>MGSSHHHHHHSSGENLYFQGHMMDLTVEPNLHSLITSTTHKWIFVGGKGGVGKTTSSCSIAIQMALSQPNKQFLLISTNPAHNLSDAFGEKFGKDARKVTGMNNLSCMEIDPSAALKDMNDMAVSRANNNGSDGQGDDLGSLLQGGALADLTGSIPGIDEALSFMEVMKHIKRQEQGEGETFDTVIFDTAPTGHTLRFLQLPNTLSKLLEKFGEITNKLGPMLNSFMGAGNVDISGKLNELKANVETIRQQFTDPDLTTFVCVCISEFLSLYETERLIQELISYDMDVNSIIVNQLLFAENDQEHNCKRCQARWKMQKKYLDQIDELYEDFHVVKMPLCAGEIRGLNNLTKFSQFLNKEYNPITDGKVIYELEDKE[2x];>[2x]MVPAESNAVQAKLAKTLQRFENKIKAGDYYEAHQTLRTIANRYVRSKSYEHAIELISQGALSFLKAKQGGSGTDLIFYLLEVYDLAEVKVDDISVARLVRLIAELDPSEPNLKDVITGMNNWSIKFSEYKFGDPYLHNTIGSKLLEGDFVYEAERYFMLGTHDSMIKYVDLLWDWLCQVDDIEDSTVAEFFSRLVFNYLFISNISFAHESKDIFLERFIEKFHPKYEKIDKNGYEIVFFEDYSDLNFLQLLLITCQTKDKSYFLNLKNHYLDFSQAYKSELEFLGQEYFNIVAPKQTNFLQDMMSGFLGGSKSGGGGGENLYFQGGSSHHHHHH;>MSTSASGPEHEFVSKFLTLATLTEPKLPKSYTKPLKDVTNLGVPLPTLKYKYKQNRAKKLKLHQDQQGQDNAAVHLTLKKIQAPKFSIEHDFSPSDTILQIKQHLISEEKASHISEIKLLLKGKVLHDNLFLSDLKVTPANSTITVMIKPNPTISKEPEAEKSTNSPAPAPPQELTVPWDDIEALLKNNFENDQAAVRQVMERLQKGWSLAK[2x]

The Guided Entry of Tail-Anchored Proteins (GET) pathway ensures accurate targeting of Tail-Anchored proteins (TAs)—a diverse class of membrane proteins—to the endoplasmic reticulum (ER) membrane. In yeast, newly synthesized TAs are captured by Sgt2 and transferred to Get3 for delivery to the ER, where they undergo subsequent membrane insertion. Efficient and protected handoff of hydrophobic TAs from Sgt2 to Get3 is facilitated by the Get4/5 complex, which is thought to act as a scaffold to position TA-bound Sgt2 and Get3 in proximity while trapping Get3 in an ATP-bound conformation necessary for TA binding. For Get3 to receive the TA, it must adopt a closed, nucleotide-bound conformation, which forms a hydrophobic chamber capable of accommodating the TA's transmembrane domain.

Here, we report the 3.2 Å cryo-EM structure of the Saccharomyces cerevisiae Get3-Get4/5 complex, using full-length Get4/5 containing the Sgt2-binding domain. As previous studies have shown that ATP-bound Get3 exhibits the highest affinity for Get4/5 (22), we utilized the Get3(D57N) variant. Mutation of this residue has been previously shown to effectively trap Get3 in its ATP-bound state by allowing ATP binding without subsequent hydrolysis. The complex adopts a two-fold symmetric arrangement, with a central Get3(D57N) dimer in an ATP-bound closed conformation, flanked by two opposing Get4/5 heterodimer arms extending outward. Each Get3(D57N) monomer engages a Get4/5 heterodimer through three distinct interaction surfaces, mirrored symmetrically on the opposite side of the dimer, resulting in six contact points across the assembly. Key catalytic and nucleotide-coordinating elements in the ATPase domain, including P-loop residues K26, T32, and T33, as well as the catalytic residue D57 (mutated to N in this study), adopt conformations compatible with ATP binding and hydrolysis, indistinguishable from those observed in Get3 alone. Most notably, a region we designate as the lateral gate, which forms part of the wall of the TA-binding chamber and adopts an α-helical conformation in free Get3, undergoes a helix-to-coil transition upon Get4/5 binding. In our structure, this region is unstructured and engaged by Get4/5, creating two lateral openings on opposite sides of the chamber that increase solvent and presumably substrate accessibility. At the same time, the apical surface of the TA-binding chamber, which is typically disordered and unresolved in structures lacking Get4/5, becomes more stable and interacts with a C-terminal α-helix from Get4 to form a composite lid over the chamber. In our cryo-EM structure of the yeast Get3-Get4/5 complex, we identified a consistent density feature adjacent to the lateral gate of Get3, extending from the last modeled C-terminal residue of Get5.> MRQKRKGDLSPAELMMLTIGDVIKQLVEAHEQGKDVDLNKMKTKTAAKYGLASQPRLVDIIAAVPPHYRKILIPKLKAKPVRTASGIAVVAVMCKPHRCPHISFTGNICIYCPGGPDSDFEYSTQSYTGYEPTSMRAIRARYDPFLQTRHRIEQLKQLGHSVDKVEFIVMGGTFMALPEEYRDYFIRSLHDALSGHTSNNIHEAIKYSERSFTKCVGITIETRPDYCMKRHLSDMLTYGCTRLEIGVQSVYEDVARDTNRGHTVKAACESFHLAKDSGFKVVTHMMPDLPNVGLERD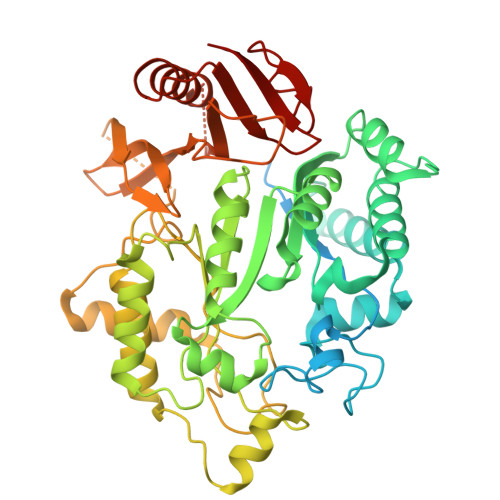IEQFIEFFENPAFRPDGLKLYPTLVIRGTGLYELWKSGRYRSYSPSDLIELVARILALVPPWTRVYRVQRDIPMPLVSSGVEHGNLRELAFARMKDLGIQCRDVRTREVGIQEIHHRVRPYQVELVRRDYVANGGWETFLSYEDPDQDILIGLLRLRKCSEETFRFELGGGVSIVRELHVYGSVVPVSSRDPTKFQHQGFGMLLMEEAERIAREEHGSGKMAVISGVGTRNYYRKIGYRLQGPYMVKMLK>[32x]KSGKPSGEMDEVGVQKCKNALKLPVLEVLPGGGWDNLRNVDMGRVMELTYSNCRTTEDGQYIIP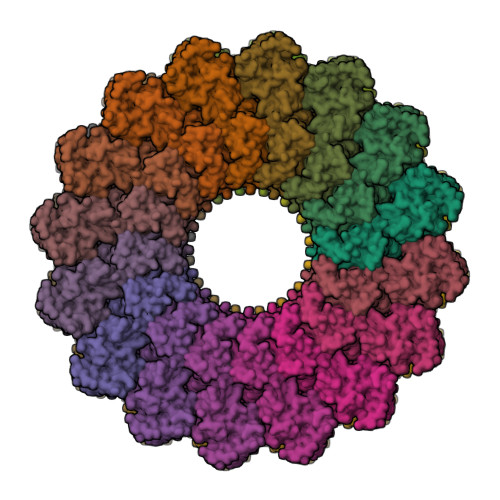DEIFTIPQKQSNLEMNSEILESWANYQSSTSYSINTELSLFSKVNGKFSTEFQRMKTLQVKDQAITTRVQVRNLVYTVKINPTLELSSGFRKELLDISDRLENNQTRMATYLAELLVLNYGTHVTTSVDAGAALIQEDHLRASFLQDSQSSRSAVTASAGLAFQNTVNFKFEENYTSQNVLTKSYLSNRTNSRVQSIGGVPFYPGITLQAWQQGITNHLVAIDRSGLPLHFFINPNMLPDLPGPLVKKVSKTVETAVKRYYTFNTYPGCTDLNSPNFNFQANTDDGSCEGKMTNFSFGGVYQECTQLSGNRDVLLCQKLEQKNPLTGDFSCPSGYSPVHLLSQIHEEGYNHLECHRKCTLKVFCKTVCEDVFQVAKAEFRAFWCVASSQVPENSGLLFGGLFSSKSINPMTNAQSCPAGYFPLRLFENLKVCVSQDYELGSRFAVPFGGFFSCTVGNPLVDPAISRDLGAPSLKKCPGGFSQHPALISDGCQVSYCVKSGLFTGGSLPPARLPPFTRPPLMSQAATNTVIVTNSENARSWIKDSQTHQWRLGEPIELRRAMNVIHGDGGGLSHHHHHH1-deoxy-1-(7,8-dimethyl-2,4-dioxo-3,4-dihydrobenzo[g]pteridin-10(2H)-yl)-3-O-phosphono-D-ribitol 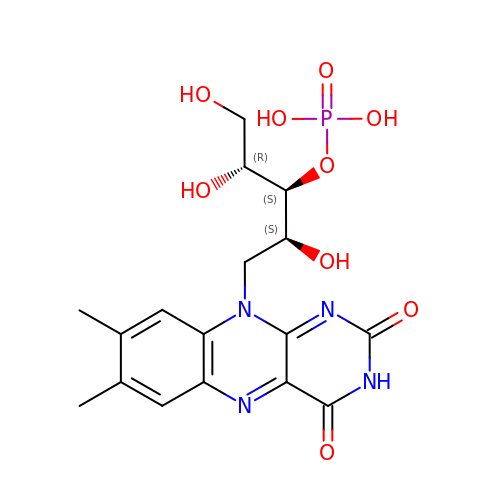| C17 H21 N4 O9 P | XTUPYSORVVXTTQ-AOUZGSJDSA-N KHNYN is a ZAP-binding protein required for ZAP-restriction of CpG-rich viral genomes. It contains an extended diKH, PIN nuclease, and CUElike domain, each of which are required for ZAP restriction of viral replication. Our crystal structure reveals an extended PIN domain (ex-PIN) containing a conserved N-terminal arm region required for domain stability and an active site tetra-Asp motif, which are both required for antiviral activity. Unlike the weak activity recently reported for the PIN domain, we demonstrate that the KHNYN ex-PIN domain is a highly active Mn2+-dependent single-stranded RNA endonuclease that cleaves with a preference for ApC, ApA, and UpA dinucleotides.

Therefore, to understand the contribution of this N-terminal extension to protein folding, stability, and catalysis, we determined the ex-PIN crystal structure that includes the N-terminal extension sequence. Within the structure, residues encompassing T411–P594 were well ordered, which includes residues T411–D436 of the N-terminal extension. The asymmetric unit comprised two copies of the ex-PIN that pack to bury a surface area of 446 Å2, although there is no indication of dimerization for the ex-PIN at up to 2 mg ml−1 concentration in solution as determined by SEC-MALLS. The domain comprises a mixed α/β fold containing nine α-helices and six β-strands. The ex-PIN N-terminal sequence forms an N-terminal arm (Nt-Arm) comprising a short helix, α1 and an extended strand that packs against the core PIN domain. Further secondary structures are arranged in two helical subdomain wings (α2–α5 and α6–α8), a central β-sheet (β1–β4), small orthogonal sheet (β5–β6), and a C-terminal short helix, α9. The copies structurally superpose well with a RMSD of 1.4 Å over 167 of 183 Cα positions but with two local conformational differences. The first in the large loop that intersperses β3 and α6 that is disordered in Monomer-A. The second in the (α6–α8) helical wing, where in Monomer-A α7 is disordered and α8 is rotated by 25° relative to its position in Monomer-B. The Nt-Arm contains 20 residues (K417–D436) that wrap around the core PIN domain. PISA analysis reveals an extensive interface that buries 890 Å2 of surface containing salt bridge, hydrogen bonds and hydrophobic interactions.

>TGTQRFKEALQDPFTLCLANVPGQPDLRHIVIDGSNVAMVHGLQHYFSSRGIAIAVQYFWDRGHRDITVFVPQWRFSKDAKVRESHFLQKLYSLSLLSLTPSRVMDGKRISSYDDRFMVKLAEETDGIIVSNDQFRDLAEESEKWMAIIRERLLPFTFVGNLFMVPDDPLGRNGPTLDEFLKKP[2x]> IVGGRRARPHAWPFMVSLQLRGGHFCGATLIAPNFVMSAAHCVANVNVRAVRVVLGAHNLSRREPTRQVFAVQRIFENGYDPVNLLNDIVILQLNGSATINANVQVAQLPAQGRRLGNGVQCLAMGWGLLGRNRGIASVLQELNVTVVTSLCRRSNVCTLVRGRQAGVCFGD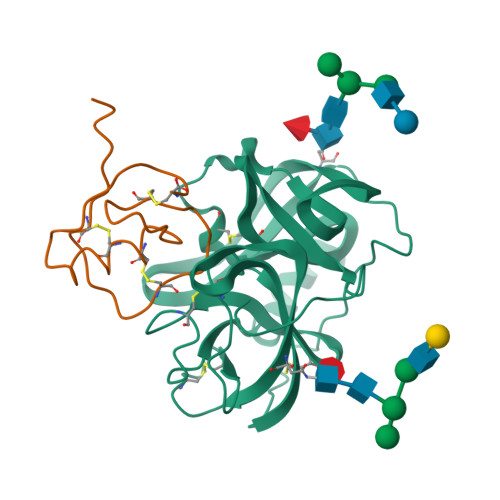SGSPLVCNGLIHGIASFVRGGCASGLYPDAFAPVAQFVNWIDSIIQ;> LAAVSVDCSEYPKPACTLEYRPLCGSDNKTYGNKCNFCNAVVESNGTLTLSHFGKC> MYGSKTFIKYVSGIPDYFKQSFPEGFTWERTTT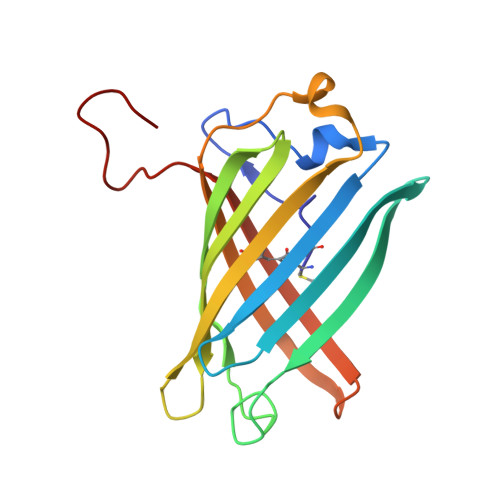YEDGGFLTAHQDTSLDGDCLVYKVKILGNNFPADGPVMQNKAGRWEPATEIVYEVDGVLRGQSLMALKCPGGRHLTCHLHTTYRSKKPASALKMPGFHFEDHRIEIMEEVEKGKCYKQYEAAVGRYCDAAPSKLGHN>TTQPALLRLSDHLLANYKKGVRPVRDWRKPTTVSIDVIMYAILNVDEKNQVLTTYIWYRQYWTDEFLQWTPEDFDNVTKLSIPTDSIWVPDILINEFVDVGKSPNIPYVYVHHRGEVQNYKPLQLVTACSLDIYNFPFDVQNCSLTFTSWLHTIQDINITLWRSPEEVRSDKSIFINQGEWELLEVFPQFKEFSIDISNSYAEMKFYVIIRRRPLFYAVSLLLPSIFLMVVDIVGFCLPPDSGERVSFKITLLLGYSVFLIIVSDTLPATAIGTPLIGVYFVVCMALLVISLAETIFIVRLVHKQDLQRPVPDWLRHLVLDRIAWILCLGEQPMAHRPPATFQANKTDDCSAMGNHCSHVG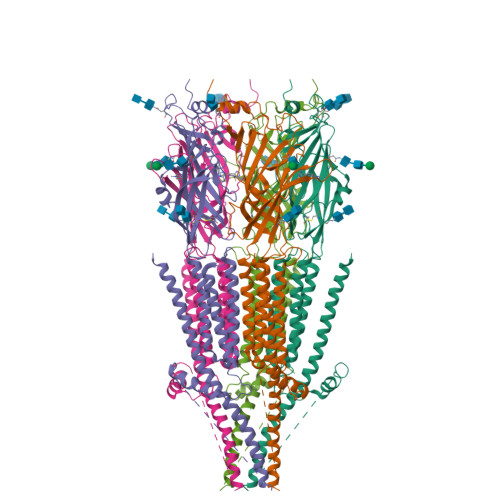GPQDLEKTPRGRGSPLPPPREASLAVRGLLQELSSIRHFLEKRDEMREVARDWLRVGYVLDRLLFRIYLLAVLAYSITLVTLWSIWHYS[5x]4-[(~{E})-(3,6-dimethyl-1,3-benzothiazol-2-yl)iminomethyl]-~{N},~{N}-dimethyl-aniline 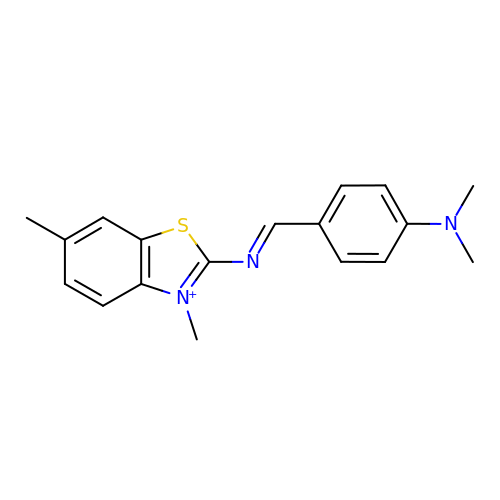| C18 H20 N3 S | YMJKNBJZXPYPNA-UHFFFAOYSA-N>[2x]AYPMPNPFPPFRIAGNLYYVGTDDLASYLIVTPRGNILINSDLEANVPMIKASIKKLGFKFSDTKILLISHAHFDHAAGSELIKQQTKAKYMVMDEDVSVILSGGKSDFHYANDSSTYFTQSTVDKVLHDGERVELGGTVLTAHLTPGHTRGCTTWTMKLKDHGKQYQAVIIGSIGVNPGAKLVDNITYPKIAEDYKHSIKVLESMRCDIFLGSHAG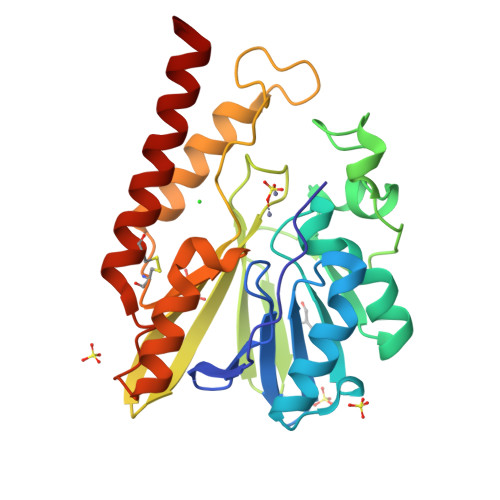MFDLKNKYVLLSKGQNNPFVDPTGCKNYIEQKANDFYTELKKQETG> MGGSVIVIDSKAAWDAQLAKGKEEHKPIVVDFTATWSGPCKMIAPLFETLSNDYAGKVIFLKVDVDAVAAVAEAAGIT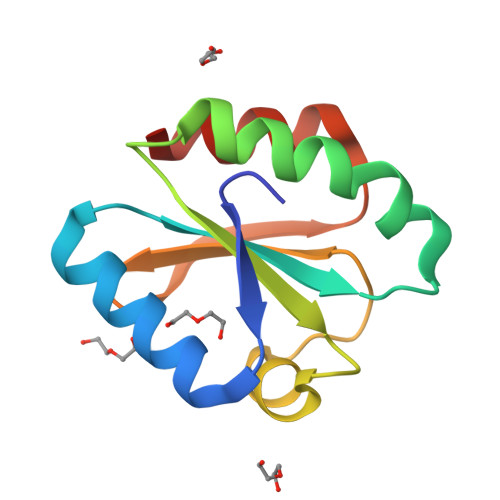AMPTFHVYKDGVKADDLVGASQDKLKALVAKHAAA>MGNIMSASFAPECTDLKTKYDSCFNEWYSEKFLKGKSVENECSKQWYAYTTCVNAALVKQGIKPALDEAREEAPFENGGKL[2x];>[2x]MGSSHHHHHHSQDPMVLLHKSTHIFPTDFASVSRAFFNRYPNPYSPHVLSIDTISRNVDQEGNLRTTRLLKKSGKLPTWVKPFLRGITETWIIEVSVVNPANSTMKTYTRNLDHTG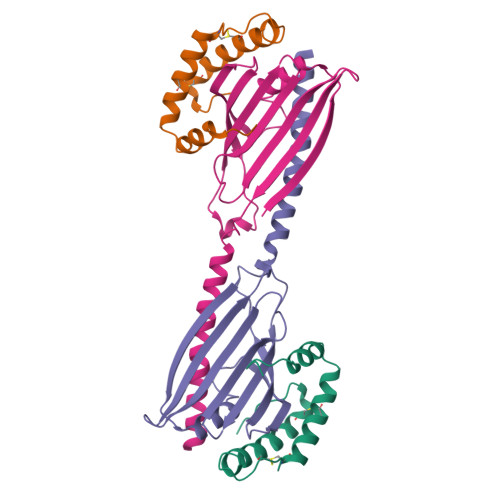IMKVEEYTTYQFDSATSSTIADSRVKFSSGFNMGIKSKVEDWSRTKFDENVKKSRMGMAFVIQKLEEA>GSPCPGACVCYNEPKVTTSCPQQGLQAVPTGIPASSQRIFLHGNRISHVPAASFQSCRNLTILWLHSNALARIDAAAFTGLTLLEQLDLSDNAQLHVVDPTTFHGLGHLHTLHLDRCGLRELGPGLFRGL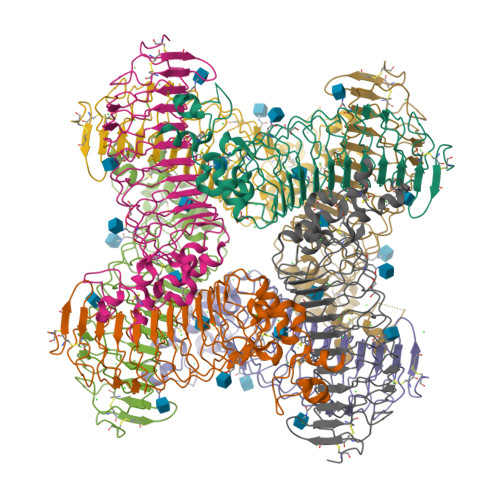AALQYLYLQDNNLQALPDNTFRDLGNLTHLFLHGNRIPSVPEHAFRGLHSLDRLLLHQNHVARVHPHAFRDLGRLMTLYLFANNLSMLPAEVLMPLRSLQYLRLNDNPWVCDCRARPLWAWLQKFRGSSSEVPCNLPQRLADRDLKRLAASDLEGCAVASGPFRPIQTSQLTDEELLSLPKCCQAAAHHHHHH[8x]>[2x]MAENTEPRIGVFVCHCGTNIAGSMSIDDVVNYAKTLPYVAVADQYQYMCSTPGQKKIDDAIKEYNLTGVVVAACSPRLHEPTFRTATKEGGLNPFRFEMANIREQNSWVHMHGMWDEATQKAKDQVRMAVAKAAKLEDLVPKSVPVEKTAMVVGGGVAGMQAALDLASAGIKTYLIERTPTIGGRMSQLDKTFPTLDCSQCILTPKMVDVGRHPNIEMMTYTEVEKVEGYIGNFDVTLRKKARGVLTPTEATAKGIVGGGCNGCGDCSAVCPVIKPNPFEMGMAPRKAIYIYHAQVMPLIYTVDFDSCVKCGLCVEACGDKKAIDLEMQDEFITVKVGTAVLATGYELFPIENKREWGYKQFDNVINALEFERLICASGPTGGHLVRPSDGKTPMKVGFVLCAGSRDNTGIGKPYCSRFCCMYSLKHAHQIMEKIPGAVAYLFYMDIRSFGKMYEEFYYRIQHEGAKFIRGRVANVLEDKETKNLHVFTEDTLLGRPVDVEVDLLVLAAAVQPNEGANELRKKFGVSASQDGWMLEAHPKLNPCGTTTAGVFLAGVCQGPKDIPDTVAQAEGAASAASIPIHMGEVELEPYFAMCIDELCAGCGMCVNLCPYSALSLGEKNGRTVMVVTEAKCKGCGTCGGFCPGGAIKMQHFTTPQIVAQIDAFFAGGEQ;>MHEYAFFLGCIAPNRYPGCEASAIKTSEKVGIKLLPLKGASCCPAPGAFGSIDLNVWYAMAARNLVLAEEMKKDIALICNGCYKSIWEVNHILKHNDELRDNVNEVLAEIDMQFKGTIDVWHLAELYYDDKVCGVQKIKDSVTTPLSGAKVAAHYGCHLMKPKKERHFGDTENPMWFEELIGALGAEPIQYRNKMQCCGAGGGVRGYDIVHALDITNEKLINIQEAGADAITELCPFCQLQFDRGQIEIKEKFGDVYNIPVLHYNELLGLAQGMSPQDLALDLHAIDCTPFLQKVL[2x];>MAAKSYNIPELDKKLADRRYHLSDTNPEFTQKILKTSRTIANMCYQCGTCTGSCPSAPRSSYRIRLFMRRCVLGLENEALTDPDLWLCTTCYSCTDRCPRDIAPTDVIMAMRNLAFKRDIVPKNFLQTVQLIYNSGHGVPNNDVNRAARTKLGLPADPPTTHSYPEFVKGIQKIIDHYELKENADRILKGD[2x];>[2x]MSENSEIMKYVATTCPYCGVGCTLNLVVSNGKVVGVEPNQRSPINEGKLCPKGVTCWEHIHSPDRLTTPLIKKDGKFIEASWDEALDLVAKNLKVIYDKHGPKGLGFQTSCRTVNEDCYIFQKFARVGFKTNNVDNCARICHGPSVAGLSLSFGSGAATNGFEDALNADLILIWGSNAVEAHPLAGRRIAQAKKKGIQIIAVDPRYTMTARLADTYVRFNPSTHIALANSMMYWIIKEGLEDKKFIQDRVNGFEDLKKTVENYADAEAIHGVPLDVVKDIAFRYAKAKNAVIIYCLGITELTTGTDNVRSMGNLALLTGNVGREGVGVNPLRGQNNVQGACDMGAYPNVYSGYQKCEVAENRAKMEKAWSVTNLPDWYGATLTEQINQCGDEIKGMYILGLNPVVTYPSSNHVKAQLEKLDFLVVQDIFFTETCQYADVILPGACFAEKDGTFTSGERRINRVRKAVNPPGQAKEDIHIISELAAKMGFKGFELPTAKDVWDDMRAVTPSMFGATYEKLERPEGICWPCPTEEHPGTPILHREKFATADGKGNLFGIDYRPPAEVADAEYPFTLMTGRLIFHYHSRTQTDRAADLHREVPESYAQINIEDARRLGIKNNEYIKLKSRRGETTTLARVTDEVAPGVVYMTMHFADGVNNLTNTVLDPMSKMPELKHCAISIEKVGGN;>MAAKGDMLYAWAKDAEIQKKGECGGAVTALLKHALETKMVDAVVAIKKGKDLYDAVP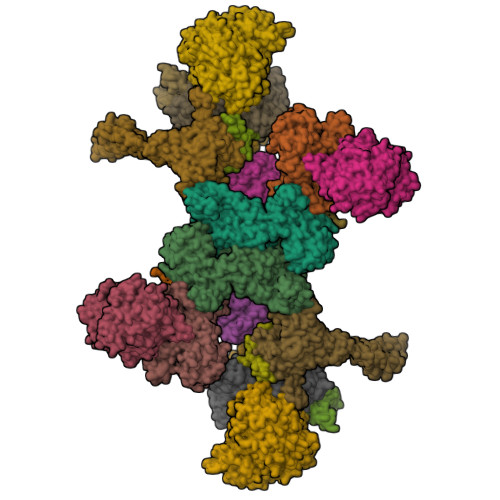TVITNPEDIIQTAGSLHCGTLLIPKLIKKYLNGAKDMKLAVTCKGCDAMAFYELAKRNQINLDNIIMIGVNCGGSVSPVTARKMISNKFGVDPDTVHKEEIDKGQFIIEYEGGHKGIKIDELEEEGYGRRSNCRRCKMKIPRQADIAAGNWGVIGDKAGKATFLEICSEKGANLVNSAQSKGALEISPADPKGIDIRAKVEKAMFNLGDEWRHRDFEGMGKGKDRLKLMMSESSKCIKCYACVEACPICYCIECSTKKPWYIAPGVLPTSFMFHLIRFAHVSDSCINCGQCEELCPMEIPNALFMHSQQVEIEKMFGHIPGQDMTPPIHAFVEEKAERARLDATGTDSIYTNIFTDE[2x];>[2x]MADDWKPQILAIICNWCSYAGADLAGGARIQYPPTVRAIRVMCTGRVDMLFILKAFVEGADGVLVSGCHFGDCHYLEGNYKAAKRMFMIKNLLRNIGLDDRRFRMTFVSASEGAKWGMVMEDVTNTIKELGPSPIKEFKK;>[2x]MSELLIKNGYIFDPISGIKGDKADIAIKDGKIVDKVSSKAQVIDASGKTVMSGGVDIHTHVSGPKVNTGRMMRPEDKFFRGSYRGGIIKQGKRMEMGFSIPSTYKTGYAYARMGYTFTNEAAMPPLLAPHVHEEFRDTPILDQAAMPVFGNNWFCFEYIKNKELENNAAYVAWLLNATKGIGIKVVNPGGTEAWAWGENCTTINDPVPYFDITPAEIVKGLIETNEYLGLPHSVHIHGNNLGNPGNYKDTLDTLRLAESYKAKNKFGREQVLHNTHIQFHSYKGTSWADFESGAKEIMDYVNANKNITCDIGQVTLDETTTMTADGPFEYHLNQLNHIKWANVDVELETGSGVVPYIYDKNIKVCGIQWAIGLELALYAKDLMRVHITTDHPNAGPFTRYPCVIKWLMSEKARKATLDTMKWKDKVIAASNIASMDRELGLYEIAMMTRAGPAKALGLAAIYGSLVKGADGNVAIYNLDANDLPSDPELIEAAFQNTAYTIKEGVVVVKDGEIIAEPHKYTLWTKVNMPENAQVMHDIKEKFTKNYTVNLENYAVFDEHVHNPRAIELDVA;>[2x]MPKVIENVGCPYCGCSCDDVRITVSDDGKDILEVENVCAIGTEIFKHGCSKDRIRLPRMRQPDGSMKDISYEEAIDWTARHLLKAKKPLMYGFGSTNCEGQAAAARVMEIAGGMLDNCATICHGPSFLAIFDNGYPSCTLGEVKNRADVIVYWGSNPAHAHPRHMSRYSIFPRGFFTGKGQKKRTVIVIDPRFTDTANVADYHLQVKQGHDYELFNAFRMVIHGHGKDLPDEVAGIKKETILEVAEIMKNARFGTTFFGMGLTHTDGRNHNIDIAISLTRDLNKISKWTIMAMRGHYNIAGPGVVWSWTFGFPYCLDLTKQNHAHMNPGETSSVDMAMRDEVDMFINIGTDAAAHFPIPAVKQLKKHPWVTIDPSINMASEISDLHIPVCICGVDVGGIVYRMDNVPIQFRKVIEPPEGVMDDETLLNKIADRMEELKAKGEA;>[2x]METITMTLVQEPELFLECYSVTPDLFAGKSLAEIADLPAHEGKIQWKLGDFFKFEGKAGETAADTKIVVNGNVRRMKRFGQQMTAGEIIINSDADMYIGGWMKGGKITVKGNADSFLGIAMEGGEILIEGDAQNHVGSAYRGDWRGMSGGLIRVKGKAGNDIGTAMTGGTIIIEGDAFIHVLTHAEGGTVIIKGDVEGRVGGQMVKGDAYILGNLLYPLPGFKKVATVEKEVDGATYTFDQFIGDLGERKEKKKGEIIYGNIFLKK;>[2x]MKAKKTLNMITQRAVEEGIAMEIGKTSRQYFDACSIIEMNEQDMKELGIMKNTNVRVKSESGEVVVKAVVGRQTCYPGLCHIRQGVWANQVVPPRTQSTGAPQYSGFPVTVEPVPNERLKTALELVQGAVGMWKGDQ;>[2x]MSTLFPKYSKTTDGSKVIMEQRLLQQVNNLILDNDICTGCGICSEVCPEEAISVGAVGGVRRGLVDDAASIHVDETKCSYCGVCVIMCPFSALALKVDGEERLPILEKEGFPTYDKGTAIDQDKCVRCNICDDVCPRDAIDRDVPLFEGEDKEGLAKGQAVELKIEFKVDDEKCTKCGICGNLCEAINVLHKPFSPEIGKVEGEVIWDEAYCDGCNVCAEACPSEAIKVTRTVVGQKKLGNVNIIDEDCCTCRWCAINCPTEAITVNKIFEGEITFHAEKCPGGCSTCVDVCPANAIYLPTPKPAKDMKGQIEAKIAVNKDFCILCGACVNACPGEDIIYLRRDSVKIKGKETDLFKKIKEKLFTPRTSKVKEQPSLAGSVELKAVSQ;>[2x]MKYRGPEDKLIVFTFYKESKKKRHFFPFFLQKISYLFQNIYLYFLTTFVQSILIDQAGATNMAFAVHVNMERCTGCNNCVVACPVNALELNTVNPSSTDKIYKVINGDAVILDVKHELCAGCGICVDACPYDVIQLSGQPPQAVEA> GAGCAGCCTGTGTGGACATCA;> CCAXACA;> GGCTGCT;> 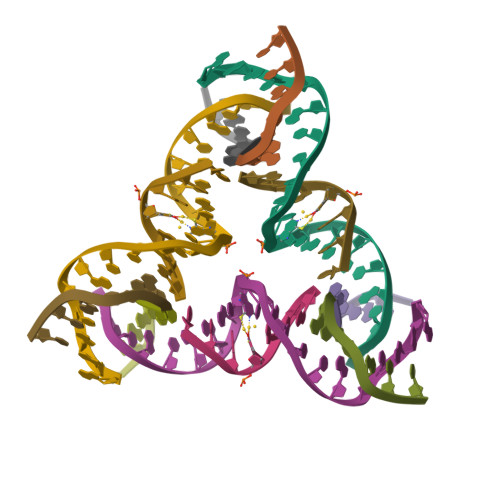CTGATGT(1R,2R,3S,4R,6S)-4,6-diamino-2-[(3-O-{2-amino-2,6-dideoxy-6-[({3-hydroxy-2-methyl-5-[(phosphonooxy)methyl]pyridin-4-yl}methyl)amino]-alpha-D-glucopyranosyl}-beta-D-ribofuranosyl)oxy]-3-hydroxycyclohexyl 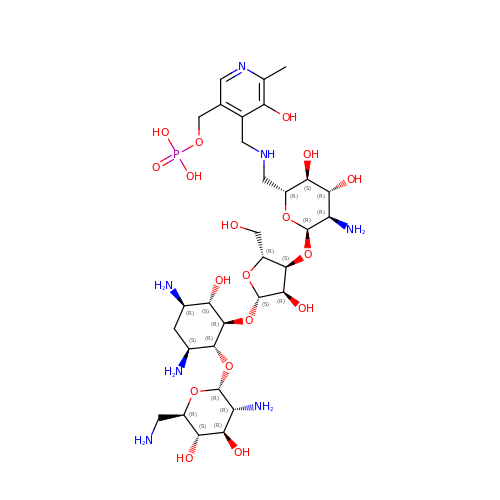2,6-diamino-2,6-dideoxy-alpha-D-glucopyranoside | C31 H56 N7 O18 P | XKWYFXMYGMVOPV-AWIIFLAXSA-N3-(methylamino)benzoic 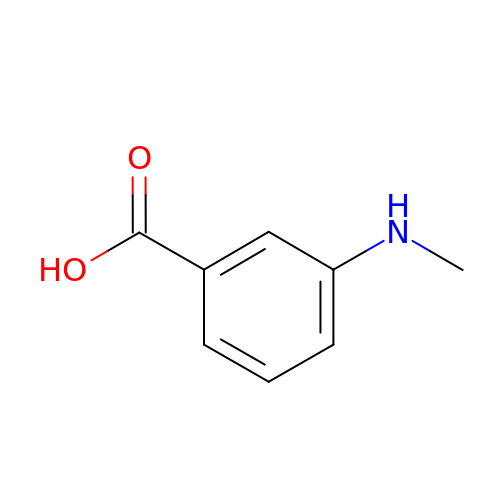acid | C8 H9 N O2 | ZCCNWBPFIBQFQX-UHFFFAOYSA-N> GSSRAMGNEVAGVEDISVEITPSSKRNSDARRTSRNCSSNEERKRRKYFHMLYLVCLMVHGFIRNEWINSKRLSRKL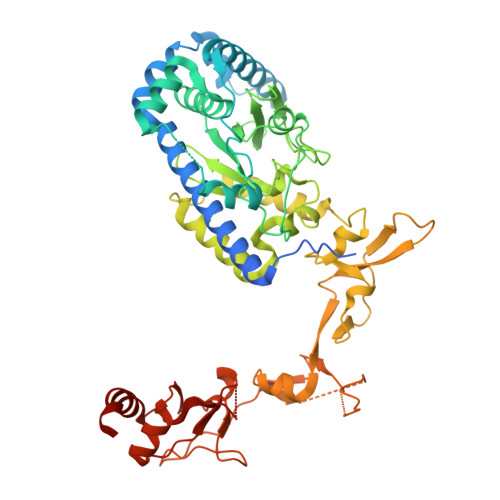SNLVPEKVFELLHPQKDEELPLRSTRKLLDGLKKCMELWQKHWKITKKYDNEGLYMRTWKEIEMSANNKRKFKTLKRSDFLRAVSKGHGDPDISVQGFVAMLRACNVNARLIMSCQPPDFTNMKIDTSLNGNNAYKDMVKYPIFWCEVWDKFSKKWITVDPVNLKTIEQVRLHSKLAPKGVACCERNMLRYVIAYDRKYGCRDVTRRYAQWMNSKVRKRRITKDDFGEKWFRKVITALHHRKRTKIDDYEDQYFFRRDESEGIPDSVQDLKNHPYYVLEQDIKQTQIVKPGCKECGYLKVHGKVGKVLKVYAKRDIADLKSARQWYMNGRILKTGSRCKKVIKRTVGRPKGEAEEEDERLYSFEDTELYIPPLASASGEITKNTFGNIEVFAPTMIPGNCCLVENPVAIKAARFLGVEFAPAVTSFKFPVLSGIVVAKWLREAIETAIDGIEFI>[2x]MEFTYSYLFRMISHEMKQKADQKLEQFDITNEQGHTLGYLYAHQQDGLTQNDIAKALQRTGPTVSNLLRNLERKKLIYRYVDAQDTRRKNIGLTTSGI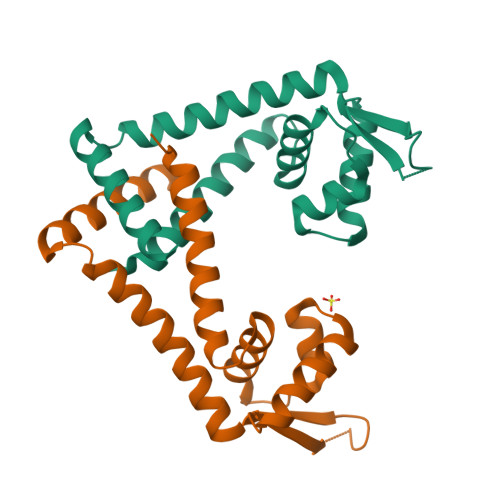KLVEVFTSIFDEMEQTLVSQLSEEENEQMKANLTKMLSSLQHHHHHH>[10x]APQNITEL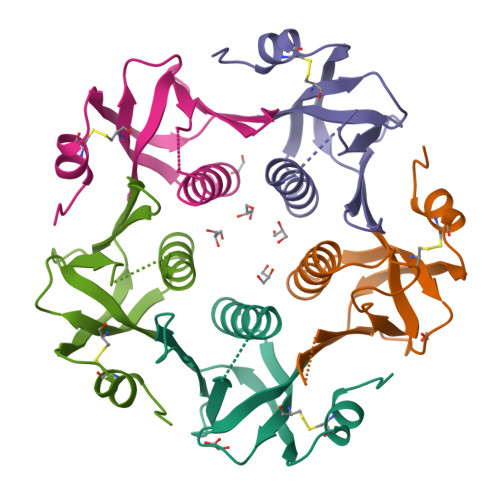CSEYHNTQIYELNKEIKTYTESLAGYREMVIISFANGATFQVEVPGSQHLESQKRPLERMKDTLRAAYFTGIKVSKLCVWNNKTPNSIAAIELSN> MATIRPDDKAIDAAARHYGITLDKTARLEWPALIDGALGSYDVVDQLYADEATPPTTSREHAVPSASENPLSAWYVTTSIPPTSDGVLTGRRVAIKDNVTVAGVPMMNGSRTVEGFTPSRDATVVTRLLAAGATVAGKAVCEDLCFSGSSFTPASGPVRNPWDRQREAGGSSGGSAALVANGDVDFAIGGDQGGSIRIPAAFCGVVGHKPTFGLVPYTGAFPIERTIDHLGPITRTVHDAALMLSVIAGRDGNDPRQADSVEAGDYLSTLDSDVDGLRIGIVREGFGHAV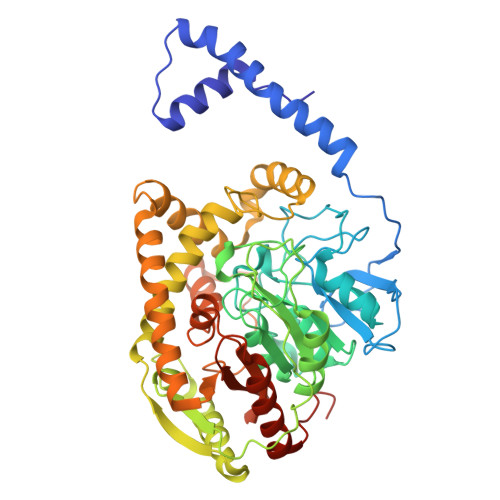SQPEVDDAVRAAAHSLTEIGCTVEEVNIPWHLHAFHIWNVIATDGGAYQMLDGNGYGMNAEGLYDPELMAHFASRRIQHADALSETVKLVALTGHHGITTLGGASYGKARNLVPLARAAYDTALRQFDVLVMPTLPYVASELPAKDVDRATFITKALGMIANTAPFDVTGHPSLSVPAGLVNGLPVGMMITGRHFDDATVLRVGRAFEKLRGAFPTPAERASNSAPQLSPA> MLPNTELYNTIFSETRKFTRESFKEIEHLTAKLANDRVARHDFLFNNSIALISDYSGEDSNGNQLQATVTIPNEITNPKEYDPSDYPLAEDESFFKQGHKYDYLVTFRAGSLTNTYEPKTKMYKLHAALDKLMHVKQRKSRFADLWRELCAVIASLDVWYQTTNYPLRTYVKLLFHKGDEFPFYESPSQDKIIFNDKSVASILPTFVYTCCQVGTAIMSGILTHVESIVAMNHFLHCAKDSYIDEKLKIKGIGRSWYQEALHNVGRATVPVWSQFNEVIGHRTKTTSEPHFVSSTFISLRAKRAELLYPEFNEYINRALRLSKT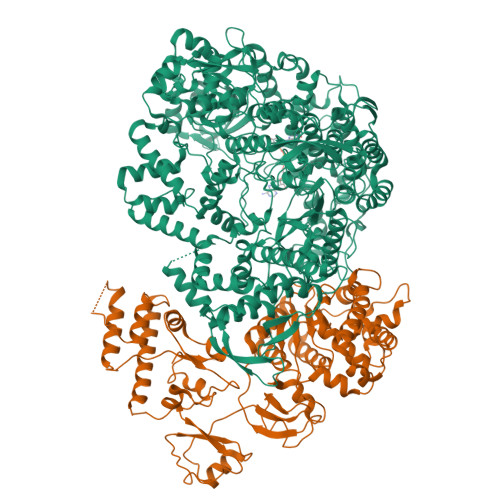QNDVANYYAACRAMTNDGTFLATLTELSLDAAVFPRIEQRLVTRPAVLMSNTRHESLKQKYANGVGSIAQSYLSSFTDEIAKRVNGIHHDEAWLNFLTTSSPGRKLTEIEKLEVGGDVAAWSNSRIVMQAVFAREYRTPERIFKSLKAPIKLVERQQSDRRQRAISGLDNDRLFLSFMPYTIGKQIYDLNDNAAQGKQAGNAFDIGEMLYWTSQRNVLLSSIDVAGMDASVTTNTKDIYNTFVLDVASKCTVPRFGPYYAKNMEVFEVGKRQSQVKYVNAAWQACALEAANSQTSTSYESEIFGQVKNAEGTYPSGRADTSTHHTVLLQGLVRGNELKRASDGKNSCLTTIKILGDDIMEIFQGNENDTHDHAVSNASILNESGFATTAELSQNSIVLLQQLVVNGTFWGFADRISLWTREDTKDIGRLNLAMMELNALIDDLLFRVRRPEGLKMLGFFCGAICLRRFTLSVDNKLYDSTYNNLSKYMTLVKYDKNPDFDSTLMSLILPLAWLFMPRGGEYPAYPFERRDGTFTEDESMFTARGAYKRRLLYDVSNIREMIQQNSMVLDDDLLHEYGFTGALLLIDLNILDLIDEVKKEDISPVKVNELATSLEQLGKLGEREKSRRAASDLKIRGHALSNDIVYGYGLQEKIQKSAMATKETTVQSKRVSSRLHEVIVAKTRDYKIPTMPADALHLYEFEVEDVTVDLLPHAKHTSYSNLAYNMSFGSDGWFAFALLGGLDRSANLLRLDVASIRGNYHKFSYDDPVFKQGYKIYKSDATLLNDFFVAISAGPKEQGILLRAFAYYSLYGNVEYHYVLSPRQLFFLSDNPVSAERLVRIPPSYYVSTQCRALYNIFSYLHILRSITSNQGKRLGMVLHPGLIAYVRGTSQGAILPEADNV;> MFAIDPLKHSKLYEEYGLYLRPHQINQEIKPTTIKKKELAPTIRSIKYASLIHSMLAKHAARHNGTLINPRMYADMITLGNTKVTVTKGTPKAQIDTLKMNGLTVVSKSRRNNKKKPVSDTTATIDENTDDIVTYKALTEMSTLIESFRLPSGLALIIFDDEKYQSLIPNYINQLIAYTQPHIIPTWQGIADFSDTYLRSYFKRPFELTASNLAAPQKYNLSPMTRSIFNNTGREDAVIRKLYGYGEYVFIRYEGCLITWTGIYGEVTMMVNLSKRDLGLDVGDDYLKEYKKLLFYGVITDAIPSGISARSTIMKISPHKMMNPSGGALAVLSKFLEAVVSTNVINATLVVYAEKGAGKTSFLSTYAEQLSLASGQVVGHLSSDAYGRWLAKNKDVEEPSFAYDYVLSLDTDDNESYYEQKASELLISHGISEVAQYELLSVRKKIKMMDEMNEVLIAQLENADTHSERNFYYMVSTGKTTPRTLIVEGHFNAQDATIARTDTTVLLRTINDTTQAMRDRQRGGVVQLFLRDTYYRLLPALHTTVYPFEMLESIRRWKWVH>[76x]MSATASTATQPKPLEWLNRLRANPRIPLIVAGSAAVAIVVAMVLWAKTPDYRTLFSNLSDQDGGAIVAQLTQMNIPYRFANGSGAIEVPADKVHELRLRLAQQGLPKGGAVGFELLDQEKFGISQFSEQVNYQRALEGELARTIETLGPVKSARVHLAMPKPSLFVREQKSPSASVTVTLEPGRALDEGQISAVVHLVSSAVAGLPPGNVTLVDQSGHLLTQSNTSGRDLNDAQLKFANDVESRIQRRIEAILSPIVGNGNVHAQVTAQLDFANKEQTEEHYSPNGDASKATLRSRQLNISEQVGAGYPGGVPGALSNQPAPPNEAPIATPPTNQQNAQNTPQTSTSTNSNSAGPRSTQRNETSNYEVDRTIRHTKMNVGDIERLSVAVVVNYKTLADGKPLPLTADQMKQIEDLTREAMGFSDKRGDTLNVVNSPFSAVDN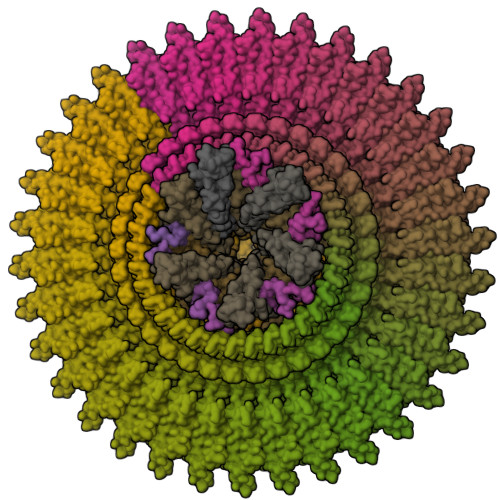TGGELPFWQQQSFIDQLLAAGRWLLVLVVAWILWRKAVRPQLTRRVEEAKAAQEQAQVRQETEEAVEVRLSKDEQLQQRRANQRLGAEVMSQRIREMSDNDPRVVALVIRQWMSNDHE;>MTPESVMMMGTEAMKVALALAAPLLLVALITGLIISILQAATQINEMTLSFIPKIVAVFIAIIVAGPWMLNLLLDYVRTLFSNLPYIIG[4x];> MIQVTSEQWLYWLHLYFWPLLRVLALISTAPILSERAIPKRVKLGLGIMITLVIAPSLPANDTPLFSIAALWLAMQQILIGIALGFTMQFAFAAVRTAGEFIGLQMGLSFATFVDPGSHLNMPVLARIMDMLAMLLFLTFNGHLWLISLLVDTFHTLPIGSNPVNSNAFMALARAGGLIFLNGLMLALPVITLLLTLNLALGLLNRMAPQLSIFVIGFPLTLTVGIMLMAALMPLIAPFCEHLFSEIFNLLADIVSEMPINNNP;>[5x]MRRLLFLSLAGLWLFSPAAAAQLPGLISQPLAGGGQSWSLSVQTLVFITSLTFLPAILLMMTSFTRIIIVFGLLRNALGTPSAPPNQVLLGLALFLTFFIMSPVIDKIYVDAYQPFSEQKISMQEALDKGAQPLRAFMLRQTREADLALFARLANSGPLQGPEAVPMRILLPAYVTSELKTAFQIGFTIFIPFLIIDLVIASVLMALGMMMVPPATIALPFKLMLFVLVDGWQLLMGSLAQSFYS;>[6x]MAAIQGIEGVISQLQATAMAARGQDTHSQSTVSFAGQLHAALDRISDRQAAARVQAEKFTLGEPGIALNDVMADMQKASVSMQMGIQVRNKLVAAYQEVMSMQV;>[5x]MLDRLDAALRFQQEALNLRAQRQEILAANIANADTPGYQARDIDFASELKKVMVRGREETGGVALTLTSSHHIPAQAVSSPAVDLLYRVPDQPSLDGNTVDMDRERTQFADNSLKYQMGLTVLGSQLKGMMNVLQGGN;>MALLNIFDIAGSALAAQSKRLNVAASNLANADSVTGPDGQPYRAKQVVFQVDAAPGQATGGVKVASVIESQAPEKLVYEPGNPLADANGYVKMPNVDVVGEMVNTMSASRSYQANIEVLNTVKSMMLKTLTLGQ[6x]> MALSKSMHARNRYKDKPPDFAYLASKYPDFKQHVQINLNGRVSLNFKDPEAVRALTCTLLREDFGLSIDIPLERLIPTVPLRLNYIHWVEDLIGHQDSDKSTLRRGIDIGTGASCIYPLLGATLNGWYFLATEVDDMCFNYAKKNVEQNNLSDLIKVVKVPQKTLLMDALKEESE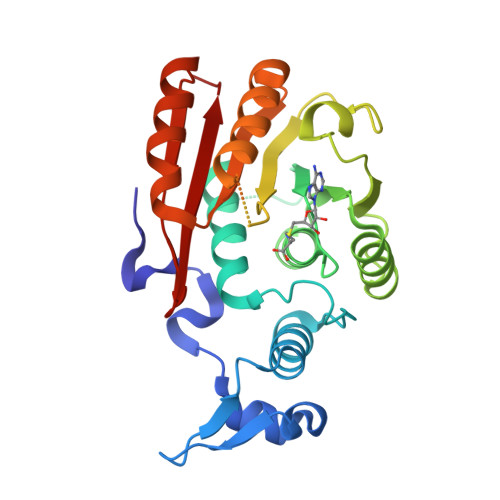IIYDFCMCNPPFFANQLEAKGVNSRNPRRPPPSSVNTGGITEIMAEGGELEFVKRIIHDSLQLKKRLRWYSCMLGKKCSLAPLKEELRIQGVPKVTYTEFCQGRTMRWALAWSFYD> MVPKLFTSQICLLLLLGLLAVEGSLHMKPPQFTWAQWFETQHINMTSQQCTNAMQVINNYQRRCKNQNTFLLTTFA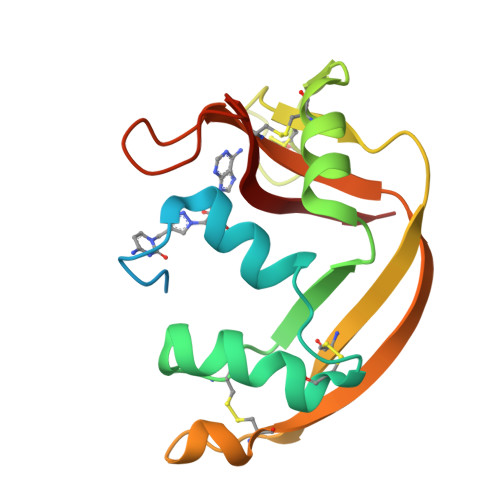NVVNVCGNPNMTCPSNKTRKNCHHSGSQVPLIHCNLTTPSPQNISNCRYAQTPANMFYIVACDNRDQRRDPPQYPVVPVHLDRII>[2x]MILVTGSSGQIGTELVPYLAEKYGKKNVIASDIVQRDTGGIKFITLDVSNRDEIDRAVEKYSIDAIFHLAGI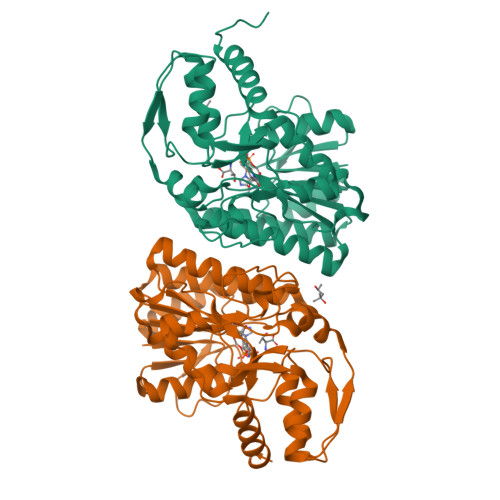LSAKGEKDPALAYKVNMNGTYNILEAAKQHRVEKVVIPSTIGVFGPETPKNKVPSITITRPRTMFGVTKIAAELLGQYYYEKFGLDVRSLRYPGIISYKAEPTAGTTDYAVEIFYYAVKREKYKCYLAPNRALPMMYMPDALKALVDLYEADRDKLVLRNGYNVTAYTFTPSELYSKIKERIPEFEIEYKEDFRDKIAATWPESLDSSEASNEWGFSIEYDLDRTIDDMIDHISEKLGIEGKHAL>GSGVGISTGGWVGGSYFTDSYVITKNTRQFLVKIQNDHKYRTENIIPSNAGGKSQRCVSTPWSYFNFNQYSSHFSPQDWQRLTNEYKRFKPRKMHVKIYNLQIKQILSNGADTTYNNDLTAGVHIFCDGEHAYPNATHPWDEDVMPELPYETWYLFQYGYIPVIHELAEMEDANAVEKAIALQIPFFMLENSDHEVLRTGESTEFTFDFDCEWINNERAYIPPGLMFNPKVPTRRAQYIRQHGNTASSNTRIQPYAKPTSWMTGPGLLSAQRVGPAGSDTASWMVVVNPDGTAVNSGMAGVG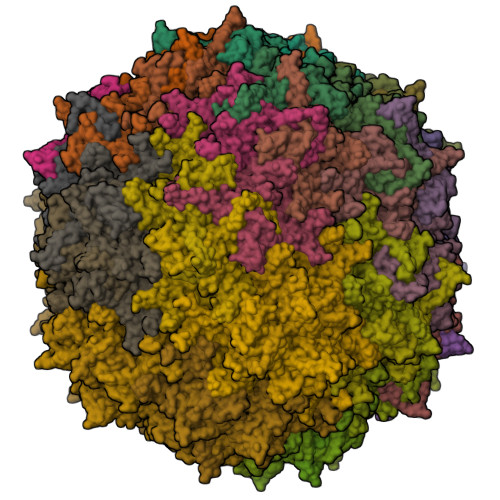SGFDPPSGSLRPTDLEYKIQWYQTPEGTNSDGNIISNPPLSMLRDQALYRGNQTTYNLCSDVWMFPNQIWDRYPITRENPIWCKKPRSDKNTIIDPFDGTLAMDHPPGTIFIKMAKIPVPSNNNADSYLNIYCTGQVSCEIVWEVERYATKNWRPERRHTALGLGIGGEENINPTYHVDKNGKYIQPTTWDMCYPIKTNINKVL[60x]>[2x]GAEFKLSDSKTSNIESVPIYSIDEFFLQRKLRSELGYKDTSVIQDLSEKILNDIETLEHNPVALEQKLVDLLKFENISLAEFILKNRSTIFWGIRLAKSTENEIPNLIEKMVAKGLNDLVEQYKFRETTHSKRELDSGDDQPQSSEAKRTKFSNPAIPPVIDLEKIKFDESSKLMTVTKVSLPEGSFKRVKPQYDEIHIPAPSKPVIDYEL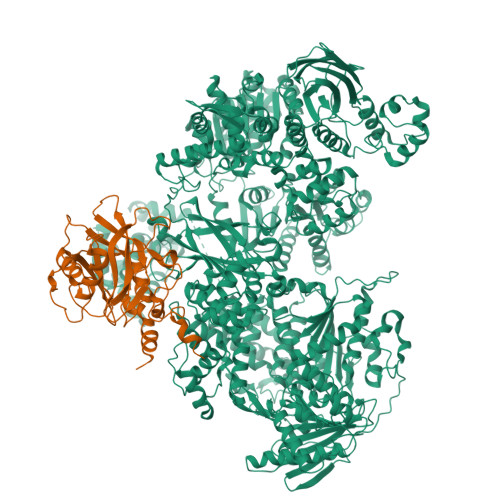KEITSLPDWCQEAFPSSETTSLNPIQSKVFHAAFEGDSNMLICAPTGSGKTNIALLTVLKALSHHYNPKTKKLNLSAFKIVYIAPLKALVQEQVREFQRRLAFLGIKVAELTGDSRLSRKQIDETQVLVSTPEKWDITTRNSNNLAIVELVRLLIIDEIHLLHDDRGPVLESIVARTFWASKYGQEYPRIIGLSATLPNYEDVGRFLRVPKEGLFYFDSSFRPCPLSQQFCGIKERNSLKKLKAMNDACYEKVLESINEGNQIIVFVHSRKETSRTATWLKNKFAEENITHKLTKNDAGSKQILKTEAANVLDPSLRKLIESGIGTHHAGLTRSDRSLSEDLFADGLLQVLVCTATLAWGVNLPAHTVIIKGTDVYSPEKGSWEQLSPQDVLQMLGRAGRPRYDTFGEGIIITDQSNVQYYLSVLNQQLPIESQFVSKLVDNLNAEVVAGNIKCRNDAVNWLAYTYLYVRMLASPMLYKVPDISSDGQLKKFRESLVHSALCILKEQELVLYDAENDVIEATDLGNIASSFYINHASMDVYNRELDEHTTQIDLFRIFSMSEEFKYVSVRYEEKRELKQLLEKAPIPIREDIDDPLAKVNVLLQSYFSQLKFEGFALNSDIVFIHQNAGRLLRAMFEICLKRGWGHPTRMLLNLCKSATTKMWPTNCPLRQFKTCPVEVIKRLEASTVPWGDYLQLETPAEVGRAIRSEKYGKQVYDLLKRFPKMSVTCNAQPITRSVMRFNIEIIADWIWDMNVHGSLEPFLLMLEDTDGDSILYYDVLFITPDIVGHEFTLSFTYELKQHNQNNLPPNFFLTLISENWWHSEFEIPVSFNGFKLPKKFPPPTPLLENISISTSELGNDDFSEVFEFKTFNKIQSQVFESLYNSNDSVFVGSGKGTGKTAMAELALLNHWRQNKGRAVYINPSGEKIDFLLSDWNKRFSHLAGGKIINKLGNDPSLNLKLLAKSHVLLATPVQFELLSRRWRQRKNIQSLELMIYDDAHEISQGVYGAVYETLISRMIFIATQLEKKIRFVCLSNCLANARDFGEWAGMTKSNIYNFSPSERIEPLEINIQSFKDVEHISFNFSMLQMAFEASAAAAGNRNSSSVFLPSRKDCMEVASAFMKFSKAIEWDMLNVEEEQIVPYIEKLTDGHLRAPLKHGVGILYKGMASNDERIVKRLYEYGAVSVLLISKDCSAFACKTDEVIILGTNLYDGAEHKYMPYTINELLEMVGLASGNDSMAGKVLILTSHNMKAYYKKFLIEPLPTESYLQYIIHDTLNNEIANSIIQSKQDCVDWFTYSYFYRRIHVNPSYYGVRDTSPHGISVFLSNLVETCLNDLVESSFIEIDDTEAEVTAEVNGGDDEATEIISTLSNGLIASHYGVSFFTIQSFVSSLSNTSTLKNMLYVLSTAVEFESVPLRKGDRALLVKLSKRLPLRFPEHTSSGSVSFKVFLLLQAYFSRLELPVDFQNDLKDILEKVVPLINVVVDILSANGYLNATTAMDLAQMLIQGVWDVDNPLRQIPHFNNKILEKCKEINVETVYDIMALEDEERDEILTLTDSQLAQVAAFVNNYPNVELTYSLNNSDSLISGVKQKITIQLTRDVEPENLQVTSEKYPFDKLESWWLVLGEVSKKELYAIKKVTLNKETQQYELEFDTPTSGKHNLTIWCVCDSYLDADKELSFEINVK;>GAMSSKNEWRKSAIANTLLYLRLKNIYVSADDFVEEQNVYVLPKNLLKKFIEISDVKIQVAAFIYGMSAKDHPKVKEIKTVVLVPQLGHVGSVQISNIPDIGDLPDTEGLELLGWIHTQTEELKFMAASEVATHSKLFADKKRDCIDISIFSTPGSVSLSAYNLTDEGYQWGEENKDIMNVLSEGFEPTFSTHAQLLLSDRITGNFIIPSGNVWNYTFMGTAFNQEGDYNFKYGIPLEFYNEMHRPVHFLQFSELAGDEELEAEQIDVFS[2x]>[4x]MKLSGVELRRVQMPLVAPFRTSFGTQSVRELLLLRAVTPAGEGWGECVTMAGPLYSSEYNDGAEHVLRHYLIPALLAAEDITAAKVTPLLAKFKGHRMAKGALEMAVLDAELRAHERSFAAELG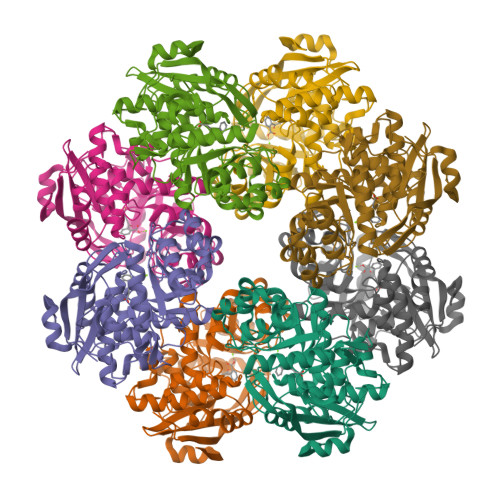SVRDSVPCGVSVGIMDTIPQLLDVVGGYLDEGYVRIKLKIEPGWDVEPVRAVRERFGDDVLLQVDANTAYTLGDAPQLARLDPFGLLLIEQPLEEEDVLGHAELARRIQTPICLDESIVSARAAADAIKLGAVQIVNIKPGRVGGYLEARRVHDVCAAHGIPVWCGGMIETGLGRAANVALASLPNFTLPGDTSASDRFYKTDITEPFVLSGGHLPVPTGPGLGVAPIPELLDEVTTAKVWIGS>[2x]GEDEIESAGVSASEVESSATKQKVALH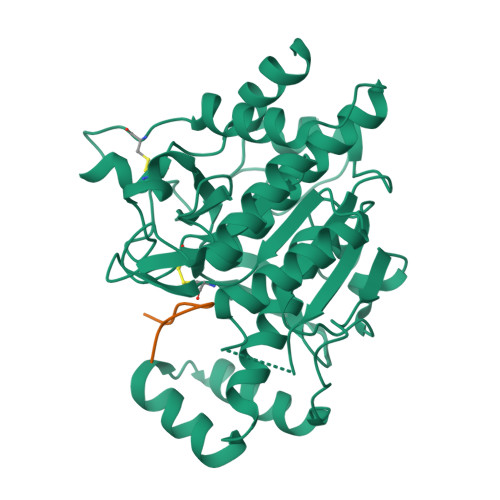PHDLDERIPGLADLHNQTLGDPQITIVIIDGDPDYTLSCFEGAEVSKVFPYWHEPAEPITPEDYAAFQSIRDQGLKGKEKEEALEAVIPDTKDRIVLNDAACHVTSTIVGQEHSPVFGIAPNCRVINMPQDAVIRGNYDDVMSPLNLARAIDLALELGANIIHCAFCRPTQTSEGEEILVQAIKKCQDNNVLIVSPTGNNSNESWCLPAVLPGTLAVGAAKVDGTPCHFSNWGGNNTKEGILAPGEEILGAQPCTEEPVRLTGTSMAAPVMTGISALLMSLQVQQGKPVDAEAVRTALLKTAIPCDPEVVEEPERCLRGFVNIPGAMKVLFGQ;> VGAPIPFPAYDG> GPM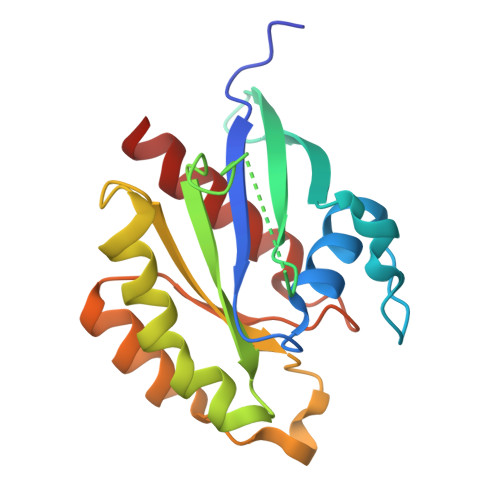PEYDYLFKLLLIGDSGVGKSCLLLRFADDTYTESYISTIGVDFKIRTIELDGKTIKLQIWDTAGQERFRTITSSYYRGAHGIIVVYDVTDQESYANVKQWLQEIDRYASENVNKLLVGNKSDLTTKKVVDNTTAKEFADSLGIPFLETSAKNATNVEQAFMTMAAEIKKRMG>MGSDKIHHHHHHVDALEVHRFLKGKIRTALPVEKVDRETLSLLYTPGVADVARACAEDPEKTYVYTSRWNTVAVVSDGSAVLGLGNIGPYGALPVMEGKAFLFKAFADIDAFPICLSESEEEKIISIVKSLEPSFGGINLEDIGAPKCFRILQRLSEEMNIPVFHDDQQGTAVVVSAAFLNALKLTEKKIEEVKVVVNGIGAAGYNIVKFLLDLGVKNVVAVDRKGILNENDPETCLNEYHLEI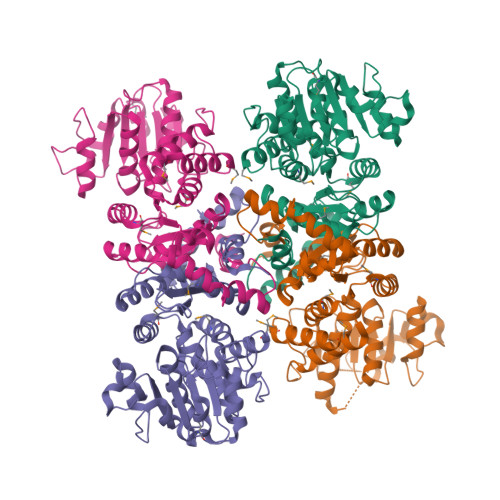ARITNPERLSGDLETALEGADFFIGVSRGNILKPEWIKKMSRKPVIFALANPVPEIDPELAREAGAFIVATGRSDHPNQVNNLLAFPGIMKGAVEKRSKITKNMLLSAVEAIARSCEPEPERIIPEAFDMKVHLNVYTAVKGSA[4x]> GSTIDSISNGILN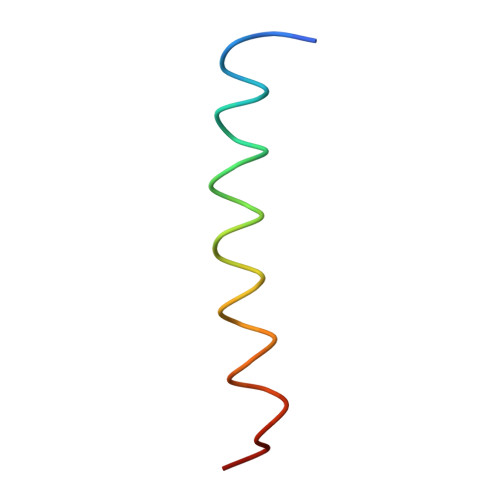NLLTTLIQDIVARETT> GAMGGSGNPLEKPPIEIVKQGREAVINYFKSLEGEKKPLNEVKVLLVGDGEAGKTSLLKRLLGEGFDGNEHQTQGINIKKWGFKDKDKEIKVNFWDFGGQEIMHA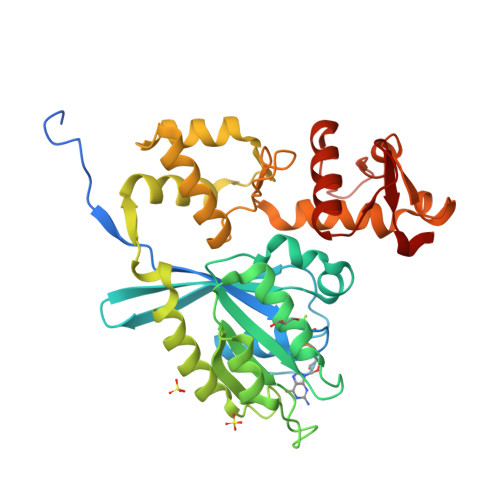THQFFLSKRSLYILVLDSRRDEKAEYWLKHIRSFGGDSPVLVALNKIDENPSFELNRKFLQEKYPSIKGFFRISCKEDRGIEGFSQKLKKELLKVEHMQIEWAKSWFEVKTKLEKMSCNFITYEEYRNICLEENVGDKSSQNTLVDFLNDLGVIVHFKDISLLDTHVLEPKWITEGVYKIINSEILAKKKGVLRFSMLDEILEQKKEGDYYYPPERYGYIINLMKKFELCYSIDEETVLLPDLL>MGSDKIHHHHHHERMYDVTPPGVVMGLAWTAMGGSTLFVETSLRRPQDKDAKGDKDGSLEVTGQLGEVMKESARIAYTFARAFLMQHAPANDYLVTSHIHLHVPEGATPKDGPSAGCTIVTALLSLAMGRPVRQNLAM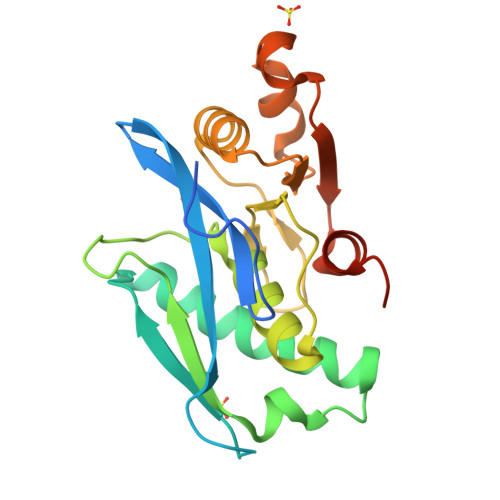TGEVSLTGKILPVGGIKEKTIAAKRAGVTCIVLPAENKKDFYDLAAFITEGLEVHFVEHYREIFDIAFPDEQAEALAVER[3x]>AMSAKDERAREILRGFKLNWMNLRDAETGKILWQGTEDLSVPGVEHEARVPKKILKCKAVSRELNFSSTEQMEKFRLEQKVYFKGQCLEEWFFEFGFVIPNSTNTWQSLIEAAPESQMMPASVLTGNVIIETKFFDDDL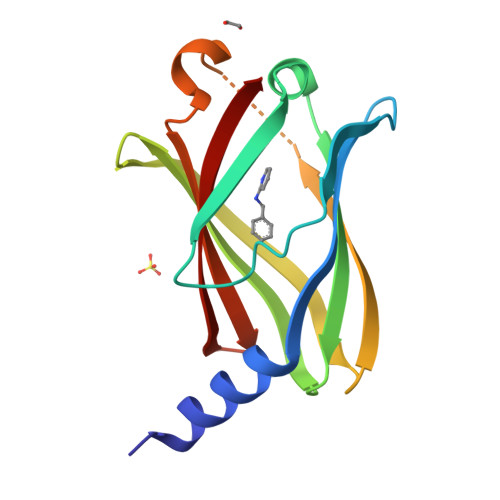LVSTSRVRLFYV[4x]>QTVPEGYQLQQVLMMSRDNLRAPLANNGSVLEQSTPNKWPEWDVPGGQLTTKGGVLEVYMGHYMREWLAEQGMVKSGECPPPYTVYAYANSLQRTVATAQFFITGAFPGCDIPVHHQEKMGTMDPTFNPVITDDSAAFSEQAVAAMEKELSKLQLTDSYQLLEKIVNYKDSPACKEKQQCSLVDGKNTFSAKYQQEPGVSGPLKVGNSLVDAFTLQYYEGFPMDQVAWGEIKSDQQWKVLSKLKNGYQDSLFTSPEVARNVAKPLVSYIDKALVTDRTSAPKITVLVGHDSNIASLLTALDFKPYQLHDQNERTPIGGKIVFQRWHDSKANRDLMKIEYVYQSAEQLRNADALTLQAPAQRVTLELSGCPIDADGFCPMDKFDSVL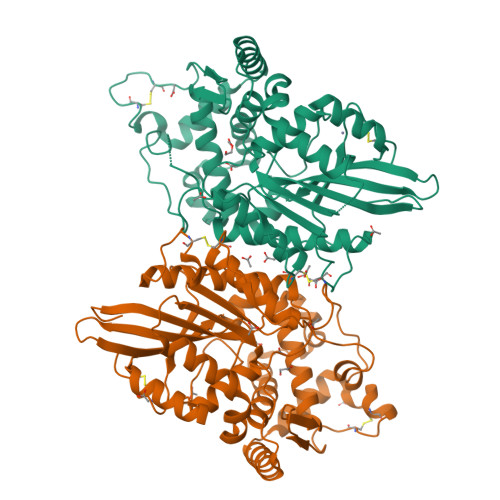NEAVK[2x]> MMDLVLEEDVTVPGTLSGCSGLVPSVPDDLDGINPNAGLGNGLLPNVSEETVSPTRARNMKDFENQITELKKENFNLKLRIYFLEERMQQEFHGPTEHIYKTNIELKVEVESLKRELQEREQLLIKASKAVESLAEAGGSEIQRVKEDARKKVQQVEDLLTKRILLLEKDVTAAQAELEKAFAGTETEKALRLRLESKLSEMKKMHEGDLAMALVLDEKDRLIEELKLSLKSKEALIQCLKEEKSQMACPDENVSSGELRGLCAAPREEKERETEAAQMEHQKERNSFQERIQALEEDLREKEREIATEKKNSLKRDKAIQGLTMALKSKEKKVEELNSEIEKLSAAFAKAREALQKAQTQEFQGSEDYETALSGKEALSAALRSQNLTKSTENHRLRRSIKKITQELSDLQQERERLEKDLEEAHREKSKGDCTIRDLRNEVEKLRNEVNEREKAMENRYKSLLSESNKKLHNQEQVIKHLTESTNQKDVLLQKFNEKDLEVIQQNCYLMAAEDLELRSEGLITEKCSSQQPPGSKTIFSKEKKQSSDYEELIQVLKKEQDIYTHLVKSLQESDSINNLQAELNKIFALRKQLEQDVLSYQNLRKTLEEQISEIRRREEESFSLYSDQTFYLSICLEENNRFQVEHFSQEELKKKVSDLIQLVKELYTDNQHLKKTIFDLSCMGFQGNGFPDRLASTEQTELLASKEDEDTIKIGEDDEINFLSDQHLQQSNEIMKDLSKGGCKNGYLRHTESKISDCDGAHAPGCLEEGAFINLLAPLFNEKATLLLESRPDLLKVVRELLLGQLFLTEQEVSGEHLDGKTEKTPKQKGELVHFVQTNSFSKPHDELKLSCEAQLVKAGEVPKVGLKDASVQTVATEGDLLRFKHEATREAWEEKPINTALSAEHRPENLHGVPGWQAALLSLPGITNREAKKSRLPILIKPSRSLGNMYRLPATQEVVTQLQSQILELQGELKEFKTCNKQLHQKLILAEAVMEGRPTPDKTLLNAQPPVGAAYQDSPGEQKGIKTTSSVWRDKEMDSDQQRSYEIDSEICPPDDLASLPSCKENPEDVLSPTSVATYLSSKSQPSAKVSVMGTDQSESINTSNETEYLKQKIHDLETELEGYQNFIFQLQKHSQCSEAIITVLCGTEGAQDGLSKPKNGSDGEEMTFSSLHQVRYVKHVKILGPLAPEMIDSRVLENLKQQLEEQEYKLQKEQNLNMQLFSEIHNLQNKFRDLSPPRYDSLVQSQARELSLQRQQIKDGHGICVISRQHMNTMIKAFEELLQASDVDYCVAEGFQEQLNQCAELLEKLEKLFLNGKSVGVEMNTQNELMERIEEDNLTYQHLLPESPEPSASHALSDYETSEKSFFSRDQKQDNETEKTSVMVNSFSQDLLMEHIQEIRTLRKRLEESIKTNEKLRKQLERQGSEFVQGSTSIFASGSELHSSLTSEIHFLRKQNQALNAMLIKGSRDKQKENDKLRESLSRKTVSLEHLQREYASVKEENERLQKEGSEKERHNQQLIQEVR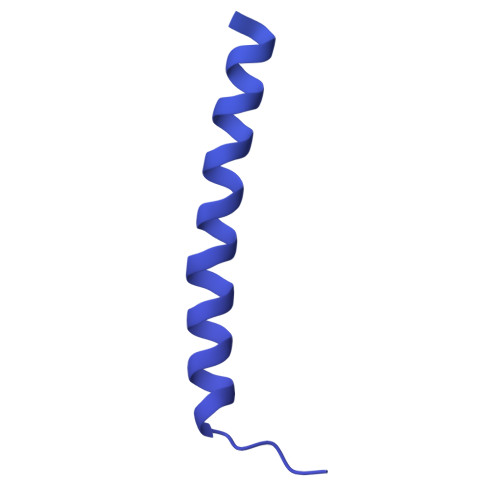CSGQELSRVQEELKLRQQLLSQNDKLLQSLRVELKAYEKLDEEHRRLREASGEGWKGQDPFRDLHSLLMEIQALRLQLERSIETSSTLQSRLKEQLARGAEKAQEGALTLAVQAVSIPEVPLQPDKHDGDKYPMESDNSFDLFDSSQAVTPKSVSETPPLSGNDTDSLSCDSGSSATSTPCVSRLVTGHHLWASKNGRHVLGLIEDYEALLKQISQGQRLLAEMDIQTQEAPSSTSQELGTKGPHPAPLSKFVSSVSTAKLTLEEAYRRLKLLWRVSLPEDGQCPLHCEQIGEMKAEVTKLHKKLFEQEKKLQNTMKLLQLSKRQEKVIFDQLVVTHKILRKARGNLELRPGGAHPGTCSPSRPGS>[14x]VLDGPYQPVAFKPPNDYWILVNSNSNGVVLEGTNNTDVWVAIIS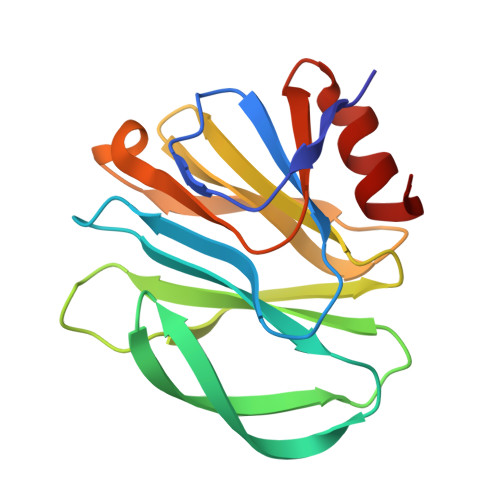IEPNVNSESRQYSLFGVNKQITVVNTSNKWKFMEMFRNNSNAEFQHKRTLTSSTKLVGILKHGGRLWTYHGETPNATTDYSTTSNLNEISVTTYAEFYIIPRSQESKCTEYINTGL> MSATKSIVGEALEYVNIGLSHFLALPLAQRISLIIIIPFIYNIVWQLLYSLRKDRPPLVFYWIPWVGSAVVYRMKPYEFFEECQKKYGDIFSFVLLGRVMTVYLGPKGHEFVFNAKLADVSAEAAYAHLTTPVFGKGVIYDCPNSRLMEQKKFVKGALTKEAFKSYVPLIAEEVYKYFRDSKNFRLNERTTGTIDVMVTQPEMTIFT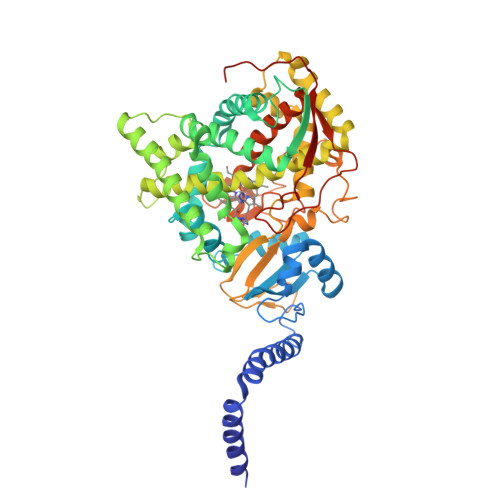ASRSLLGKEMRAKLDTDFAYLYSDLDKGFTPINFVFPNLPLEHYRKRDHAQKAISGTYMSLIKERRKNNDIQDRDLIDSLMKNSTYKDGVKMTDQEIANLLIGVLMGGQHTSAATSAWILLHLAERPDVQQELYEEQMRVLDGGKKELTYDLLQEMPLLNQTIKETLRMHHPLHSLFRKVMKDMHVPNTSYVIPAGYHVLVSPGYTHLRDEYFPNAHQFNIHRWNNDSASSYSVGEEVDYGFGAISKGVSSPYLPFGGGRHRCIGEHFAYCQLGVLMSIFIRTLKWHYPEGKTVPPPDFTSMVTLPTGPAKIIWEKRNPEQKIGGRHHHHHH> QDNSRYTHFLTQHYDAKPQGRDDRYCESIMRRRGLTSPCKDINTFIHGNKRSIKAICENKNGNPHRENLRISKSSFQVTTCKLHGGSPWPPCQYRATAGFRNVVVACENGLPVH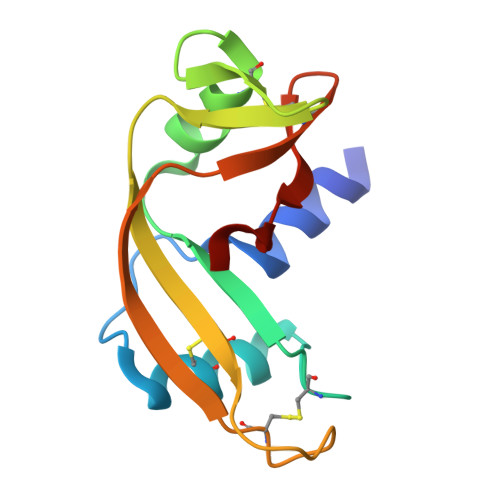LDQSAARRP>[12x]MDAAIRGNDVIFVLKTIGVPSACRQNEDPRFVEAFKCDELERYIDNNPECTLFESLRDEEAYSIVRIFMDVDLDACLDEIDYLTAIQDFIIEVSNCVARFAFTECGAIHENVIKSMRSNFSLTKSTNRDKTSFHIIFLDTYTTMDTLIAMKRTLLELSRSSENPLTRSIDTAVYRRKTTLRVVGTRKNPNCDTIHVMQPPHDNIEDYLFTYVDMNNNSYYFSLQRRLEDLVPDKLWEPGFISFEDAIKRVSKIFINSIINFNDLDENNFTTVPLVIDYVTPCALCKKRSHKHPHQLSLENGAIRIYKTGNPHSCKVKIVPLDGNKLFNIAQRILDTNSVLLTERGDHIVWIN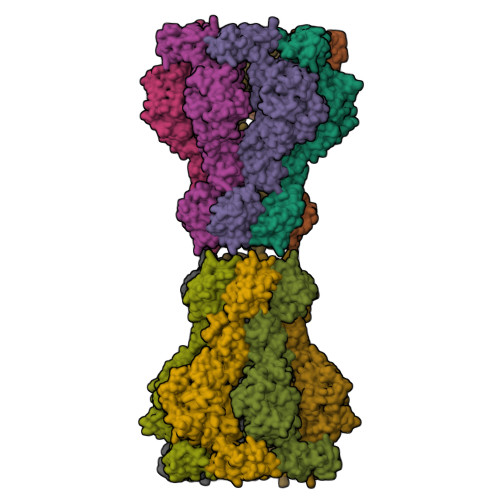NSWKFNSEEPLITKLILSIRHQLPKEYSSELLCPRKRKTVEANIRDMLVDSVETDTYPDKLPFKNGVLDLVDGMFYSGDDAKKYTCTVSTGFKFDDTKFVEDSPEMEELMNIINDIQPLTDENKKNRELYEKTLSSCLCGATKGCLTFFFGETATGKSTTKRLLKSAIGDLFVETGQTILTDVLDKGPNPFIANMHLKRSVFCSELPDFACSGSKKIRSDNIKKLTEPCVIGRPCFSNKINNRNHATIIIDTNYKPVFDRIDNALMRRIAVVRFRTHFSQPSGREAAENNDAYDKVKLLDEGLDGKIQNNRYRFAFLYLLVKWYKKYHIPIMKLYPTPEEIPDFAFYLKIGTLLVSSSVKHIPLMTDLSKKGYILYDNVVTLPLTTFQQKISKYFNSRLFGHDIESFINRHKKFANVSDEYLQYIFIEDISSP> MSKQWLCREGERWWLLDARGQQLPHVAKIAAQY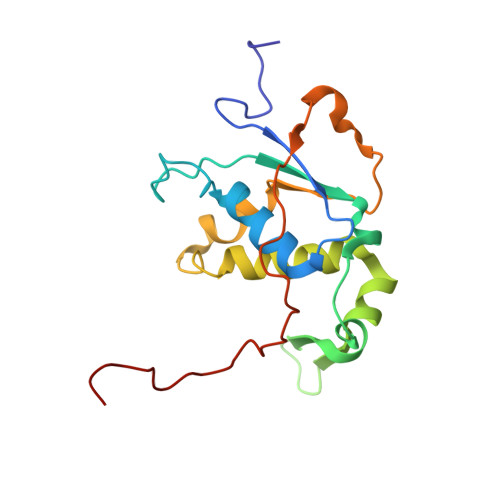MTGQHRPDFTPGMMTGDHVVITNIKDAVMTGDNWIRVPITWQTAYPGGKYRVRLSEMYERDPCMVMWWYLKDEVNRHFVRKLKTRTAPLEKAWLYEDSVHPHAEKNPRPLVWTDTATMGWRYKDPTFQRRWSPNQFMS> MDFQDYIQSLKKDFKLVKINDHTYILHKNKKTLELTPDKMYNIQEINDILNVSYPDISYDRNLEDLGSKNKGILNGFGNVGEDDLHPQIGRRKGKKKGAIFSPEEFKEEEDSDGI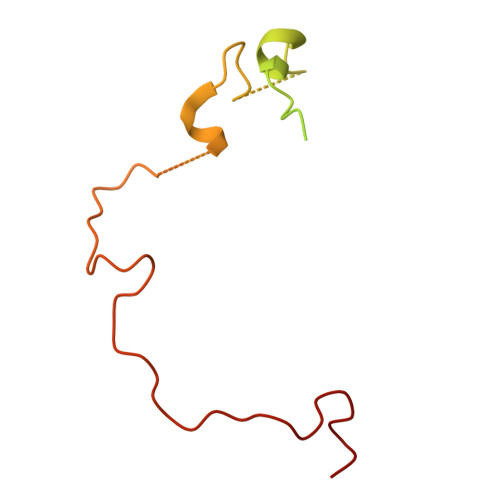DKTDIFPLKKKRDPDSDHFKKTGGDDDNPFLY> MGSSHHHHHHSQDPMDLERYAIVVSAAVEADELVLDLDKSTLEELEAKLNQELAGTDQVGEQAGKELAEGLERGAVEGLDVRQVLAKLKAALKGEVRELATEEVKALRAAIQHALGVELDDNAKRQLAESAKLLDRIIESATRNQSLTVKLRFDADRSALLTAERLADAYLNRIREALKQDKSSPLYQAFSALAKGTGEKLSPDEAKFRAGLFADVRDRFLALLKQDLQSYIADQLKRGHAVGDIKLPDTQAILSEAGLPTLKQALLLSRAVDLDANNRAKLAKDLGQFMPEVAQVLKAPEKGASWEEINAVVREAKKAIHDAEEARRVALSLRSVTKEGNKPFAQQTGRFHTIELQEEGSPDEFQELLRLQASTQGHVDETTLARLVVQKRATKAILKKLLETADRPEEQAVWRAAIERLVIGNTAYDLKDDESFAKLIELAKKHPLEKVVKNVREVQFSEKVTLSDKYAFVPASNQGRIFLSHLRRENIYRTPTQRPLSLKVAEEGEGVRLKEMEEKALGDGALGILRPQSLGLPEDYTGVVQVRGELADPEGNVYAGLKGTVIVDPRAKEDFLNLNDLYRGDTVVDGKKYTKEEVDALIREKLKTGALQLNLGIHRVSTVEEAKVGKQVFLRHMGGVPFNRGRISPSEAAKWAAQAKELKFLPMIAGREMGLSHYQQIATLAKTFGVEVDEGQYSMAASHTAYKELDPEIYRLLEEGVELDAEGRPIVPIVIGKEMAAK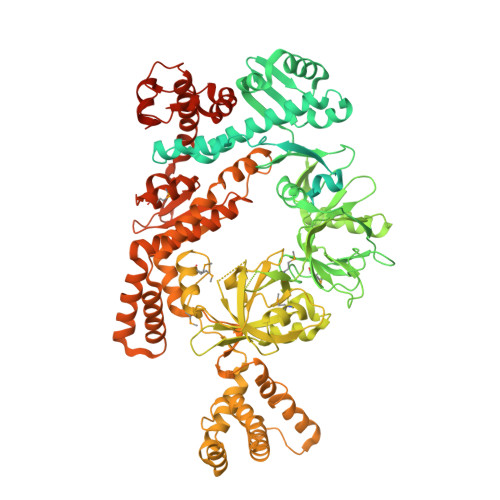LGLKEGDIAFTFRNPVMGHGGALLQARVAAIRDRLNAVVVNQEYAKSTGVDFDGDTLVVLPKGLPVDPHRLEVFQTLMAHAGLAGGRKGGGSVEPSPGELRFKEQLEVYDKVLARLSKSRLAAELRNAGVEDLSNPFEVVRQLESLGEEELLKAFKGYLRKGFAKELGLDLKSEEDRARLNQYLFEGFLDYRKQFQDPRRVYKKLPLMPSAALAASLLQVEAHKKEYDPSDPVALAAGQLTTSFLGLSEKLAQDLETSIDFPKLAEAIRAYNQAYSSGNEEQVAKARAELVKVLNDPTVQKFSLSNLLYQIITDRKKRDYSLRVRTESGKTYEYRNLYAVLNRLMQNLPVEEVADTVYDASGQAVEERVPLKQSATRSLVKGLLDLASGKVKEDPDGTVAEDLADLPVFGELEQLYGLVADAKYDPSSLKSALVKPNKPQGSYAEITTLLYRGIANQEGLAETNLPRDEVAR LCAD is a homotetramer containing one FAD per 43 kDa subunit with Glu291 as the catalytic base. LCAD substrate specificity overlaps those of VLCAD and MCAD, and in addition includes unsaturated and branched-chain substrates. Here we present the three-dimensional structure of human LCAD, revealing an unusually large substrate-binding cavity not previously reported in eucaryotic ACADs. The structural basis for the unique substrate binding cavity can be seen in the long E helix, where Pro132 is located in a position to cause unwinding of about two turns of the E helix, thus creating a large cavity.

Structures were obtained for wildtype LCAD complexed with and without acetoacetyl-CoA to 2.8 Å and 2.5 Å resolution, respectively. The first few residues at the N-terminus were not resolved in the wild type and E291Q structures. In the wild type structure, the chain starts at Glu34 (monomer A) or Leu36 (monomers B, C, and D). The C-terminal residue Lys430 is observed in all the monomers in the 2.8 Å structure of the wild type protein complexed with acetoacetyl-CoA, but not in the 2.5 Å wild type ligand-free and 2.0 Å (E291Q mutant) structures. In all LCAD structures lacking bound CoA derivatives (all eight monomers of mutant LCAD, all four monomers of ligand-free wild type LCAD, and the C and D monomers of the ligand-bound wild type LCAD), residues Ser179 through Gln182 in the vicinity of the CoA moiety of the substrate are relatively disordered in the absence of ligand. His228 and nearby residues Asp180 and Leu181 are highly mobile, judging from their weak, diffused electron densities. The side chain of Tyr282 is rotated away from the conformation of the bound structure by approximately 125 degrees.

>[4x]GGEERLETPSAKKLTDIGIRRIFSPEHDIFRKSVRKFFQEEVIPHHSEWEKAGEVSREVWEKAGKQGLLGVNIAEHLGGIGGDLYSAAIVWEEQAYSNCSGPGFSIHSGIVMSYITNHGSEEQIKHFIPQMTAGKCIGAIAMTEPGAGSDLQGIKTNAKKDGSDWILNGSKVFISNGSLSDVVIVVAVTNHEAPSPAHGISLFLVENGMKGFIKGRKLHKMGLKAQDTAELFFEDIRLPASALLGEENKGFYYIMKELPQERLLIADVAISASEFMFEETRNYVKQRKAFGKTVAHLQTVQHKLAELKTHICVTRAFVDNCLQLHEAKRLDSATACMAKYWASELQNSVAYDCVQLHGGWGYMWEYPIAKAYVDARVQPIYGGTNEIMKELIAREIVFDK Dihydropteroate synthase (DHPS, EC: 2.5.1.15) catalyses the reaction of 6-hydroxymethyl-7,8-dihydropterin-pyrophosphate with p-aminobenzoic acid (p-ABA) to yield 7,8-dihydropteroate and pyrophosphate. In so doing the enzyme supports the biosynthesis of folate, a key metabolite required to support the synthesis of DNA, and proteins. BcDHPS displays a triosephosphate isomerase (TIM)-barrel fold, consisting of eight parallel β-strands surrounded by eight α-helices. The DHPS active site is formed entirely within a single subunit.

The purified protein was used in co-crystallization screens with the inhibitor sulphadoxine or the enzyme product 7,8-dihydropteroate. However, analysis of the crystals grown in the presence of sulphadoxine revealed only water molecules in the active site and this therefore represents the apo-BcDHPS structure determined to 2.35 Å resolution. The apo-enzyme crystallized in space group C2221 with one molecule in the asymmetric unit. A number of residues could not be modeled in the electron density maps and so were omitted hence the model for this structure consists of 268 residues. Nearly 40 amino acids from each subunit participate in around 20 direct hydrogen bonds and salt bridge interactions, plus numerous water mediated contacts between the subunits and The same dimer is formed in the apo-structure by the symmetry operation -x, y, -z + ½. The first C-terminal loop, linking β1 to α1 could not be modeled in either structure, due to poorly defined density, suggesting a significant degree of conformational flexibility. Modeling of loop 2, linking β2 to α2 was possible only in the case of the product complex. The crystallographic analysis of the apo-enzyme clearly showed the normal side chains not interacting with each other.

> GHMSTFLPAPLQCGRFELTFERPLVMGILNATPDSFSDGGRFLARDDALRRAERMIAEGADLLDIGGESTRPGAPPVPLDEELARVIPLVEALRPLNVPLSIDTYKPAVMRAALAAGADLINDIWGFRQPGAIDAVRDGNSGLCAMHMLGEPQTMQVGEPDYGDVVTDVRDFLAARAQALRDAGVAAERICVDPGFGFGKAVVDDNYALLAALPDTAPARPDGRAYPILAGMSRKSMLGAVIGGKPPLERVAASVAAALCAVERGAAIVRVHDVAATVDALSVWNAVRAAARQR> SVTIDHTTENAAPAQAPVSDRAWALFRALDGKGLVPDGYVEGWKKTFEEDFSPRRGAELVARAWTDPEFRQLLLTDGTAAVAQYGYLGPQGEYIVAVEDTPTLKNVIVCSLCSCTAWPI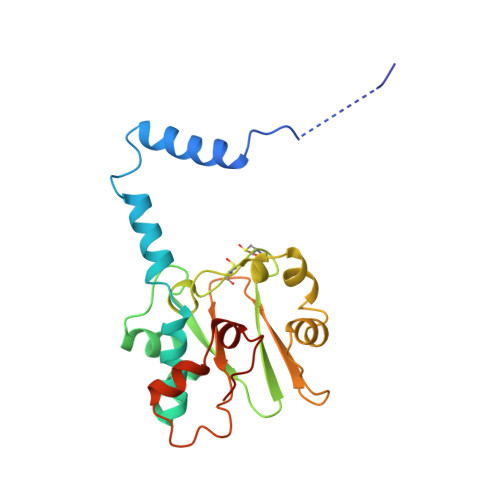LGLPPTWYKSFEYRARVVREPRKVLSEMGTEIASDIEIRVYDTTAETRYMVLPQRPAGTEGWSQEQLQEIVTKDCLIGVAIPQVPTV>[2x]MDFPQHSQHVLEQLN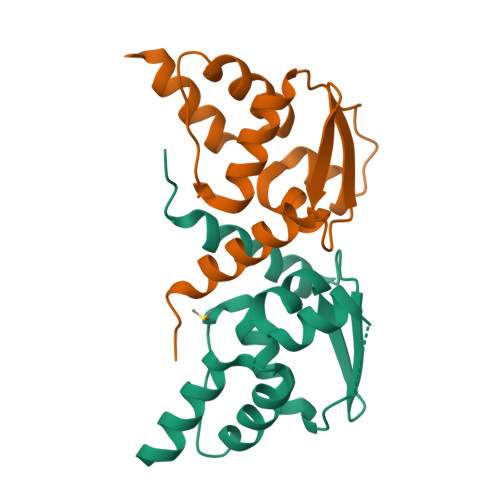QQRQLGLLCDCTFVVDGVHFKAHKAVLAACSEYFKMLFVDQKDVVHLDISNAAGLGQVLEFMYTAKLSLSPENVDDVLAVATFLQMQDIITACHALKSLA>MFRPGLEGVPATLSSISFVDGQRGVLEYRGISIEQLAQQSSFLETAYLLIWGHLPTQQELTEFEHEIRYHRRIKFRIRDMMKCFPDSGHPMDALQASAAALGLFYSRRALDDPEYIRAAVVRLLAKIPTMVAAFQLIRKGNDPIQPRDELDYAANFLYMLTEREPDPVAARIFDICLTLHAEHTINASTFSAMVTASTLTDPYAVVASAVGTLAGPLHGGANEEVLDMLEAIGSVENVEPYLDHCIATK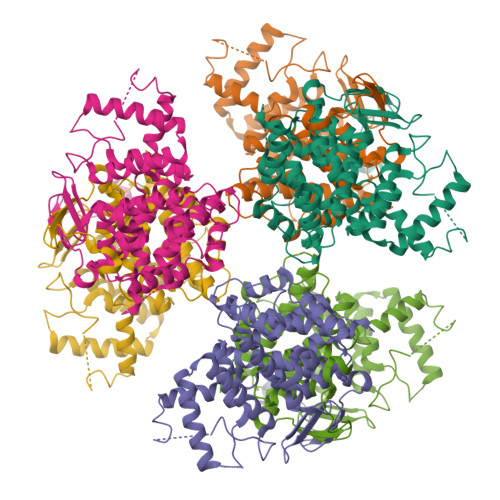TRIMGFGHRVYKVKDPRAVILQNLAEQLFDIFGHDPYYEIAVAVEKAAAERLSHKGIYPNVDFYSGLVYRKLGIPSDLFTPVFAIARVAGWLAHWKEQLNENRIFRPTQIYTGSHNLDYTPIADRDLAIESDLEHHHHHH[6x]ZER1 and ZYG11B, the substrate receptors of the Cullin 2-RING E3 ubiquitin ligase (CRL2), recognize N-terminal (Nt) glycine degrons and participate in the Nt-myristoylation quality control through the Gly/N-degron pathway. Here we show that ZER1 and ZYG11B can also recognize small Nt-residues other than glycine. Furthermore, we present the crystal structures of ZER1 and ZYG11B bound to various small Nt-residues and uncover the molecular mechanism of non-acetylated substrate recognition by ZER1 and ZYG11B. In conclusion, we propose that ZER1/ZYG11B not only targets Gly/N-degrons for proteasomal degradation, but it also has the ability to bind a defined selection of non-Ac/N-degrons by a conserved molecular mechanism of substrate recognition and target their degradation through the non-Ac/N-degron pathway.

To understand the molecular basis of ZER1/ZYG11B-mediated binding of non-Gly Nt-residue peptides, we determined the crystal structures of ZER1 bound to either SFLH-, AFLH- or TFLH-peptide, as well as the crystal structures of ZYG11B bound to either SFLH-, AFLH- or CFLH- peptide. In line with our SPOT-array results, ZER1 binds to XFLHVGQD peptides in which X is either Ser (KD of 1.3), Ala (KD of 1.6), Thr (KD of 3.1) or Cys (KD of 3.9) more potently than to the Gly-starting peptide (KD of 4.2). The free α-amino group of the Nt-residue forms hydrogen bonds with the side chains of Asp556 and Asn597 in ZER1 (the counterparts of Asp 526 and Asn 567 in ZYG11B), respectively. The main-chain amide of the third residue on the peptide is anchored by a hydrogen bond with Asn553 in ZER1 (Asn523 in ZYG11B). It is worth noting that the side-chain hydroxyl group of Nt-Ser makes additional hydrogen bond with the side chain of Trp552 in ZER1 (Trp522 in ZYG11B), suggesting a critical role of the Trp552 in binding of Nt-Ser. Apart from these direct interactions, a network of water molecules occupies the bottom of the cavity and mediates the contacts to ZER1 via water-mediated hydrogen bonds. However, on the other side, the Water3 in the Ser1-binding mode has to move down and away from the corresponding Water3 in the Gly1-binding mode (~1 Å) to provide enough space for docking the side chain of Ser1. Simultaneously, the Asn633 shifts toward Water3 to form a hydrogen bond, thereby leaving no space for Water4 in the Ser1-binding mode. As a result, the Water3 mediates contacts directly with Water2, Gly593, Asn633 as well as Ser1, while in the Gly1-binding mode the Water3 together with Water4 establishes a contact network with Water2, Gly593, Asn633 as well as Trp552. These rearrangements of water molecules might explain why ZER1 is able to recognize other Nt-residues in its narrow substrate-binding pocket.

>SFLHVGKMGFVVTMLKLIQKKLLDKTCDQVMEFSWSALWNITDETPDNCEMFLNFNGMKLFLDCLKEFPEKQELHRNMLGLLGNVAEVKELRPQLMTSQFISVFSNLLESKADGIEVSYNACGVLSHIMFDGPEAWGVCEPQREEVEERMWAAIQSWDINSRRNINYRSFEPILRLLPQGISPVSQHWATWALYNLVSVYPDKYCPLLIKEGGMPLLRDIIKMATARQETKEMARKVIEHCSNFKEENMDTSR[4x]>[4x]MNDTTAAAPGTAADPGPDAAVRALDRLIGTWRVSGGAEGTVSYRGLEGGHFLLQDIALEQFGQPVTGVEVIGRLKEFGAEEPGEDIRSRYYDSRGNTFDYVYELDGDTLTIWGGEK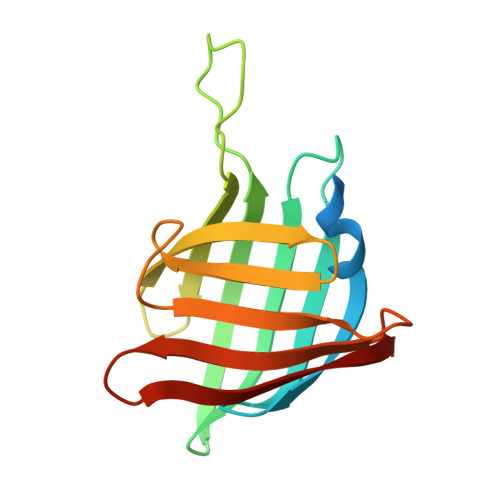GSPAYYRATFSADGNTLSGAWVYPGGGGYDSVMTRVAV> EFKHDGLISKP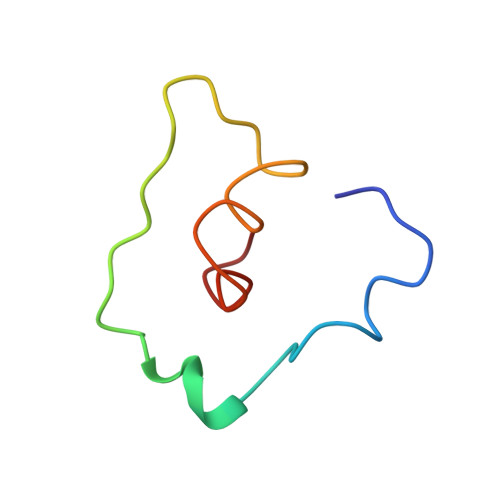ASAVAKAADALSMIPYIAPYAKATSMVADKIGKIARIFGY>MAIELWTTRNDTTSVQAFYAAEAGLQKYKAALFQQYVWREQRGGTGGGGGCFTSLARGLDLDRDGTITPFVNNRLVLAQNEVVTDANGNPVGRYTATLYKDAQDDQLFTLVSEGTSGGAKARVQATFRISNSDYLEQAIFAGAGQANKWLNGGATIRGGVYVVGNPNDPDQYVIEANGNFALYNRYDLTTYSEVTNRVEPSYRQVQDLCASLRVQYGKISVGGSTQIGEPNNKVKGVFVGRGAQDITGENVGVCRNNKGVCTEAMGGFDLSDPPPFPTLDAKLDSDACSAYPTWRACLQGKAALRIQRIGNILSVASPPNATLSPSCLQAMQSGTLTLDTQSVDCTFTRLDGSRGGFRYTYTGGQELLEVFGDVVLEGIDAVLNRPVDYRAQSGSAKSATLAVLKLGGNGGNLDINGNLLPDATFGLFPNHALGFVAEGDIYQRGQHVMAPVYAGGTFRVVKGNVLFGSVISNQFCTTSAGNQMSCNASQKAEVVYIRIPKENRPALLPSLRGGKPVFQVLSYERRLEHHHHHH[3x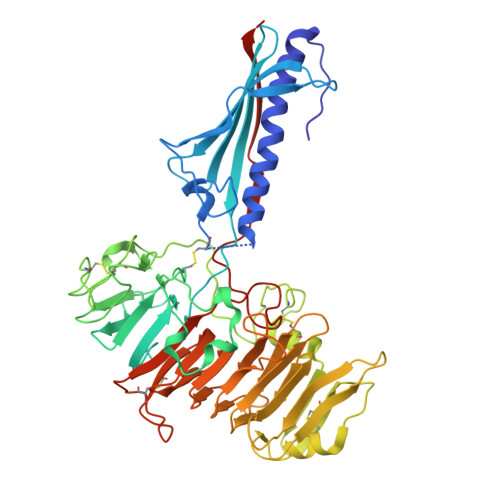]>[3x]MHHHHHHSSGLVPRGSMILHAQAKHGKPGLPWLVFLHGFSGDCHEWQEVGEAFADYSRLYVDLPGHGGSAAISVDGFDDVTDLLRKTLVSYNILDFWLVGYSLGGRVAMMAACQGLAGLCGVIVEGGHPGLQNAEQRAEAQRSDRQWVQRFLTEPLTAVFADWYQQPVFASLN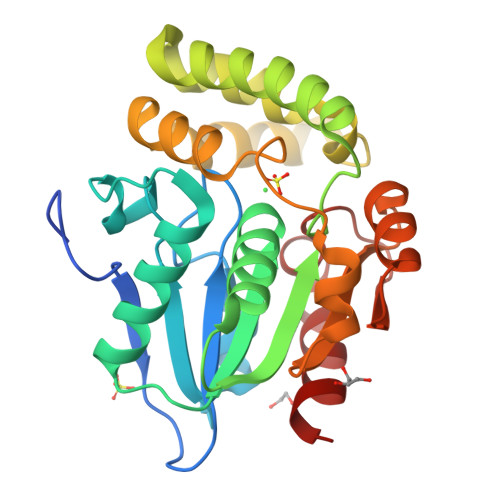DDQRRELVALRSNNNGATLAAMLEATSLAVQPDLRANLSARTFAFYYLCGERDSKFRALAAELAADCHVIPRAGHNAHRENPAGVIASLAQILRF> SLLISYESDFKTTLEQAKASLAEAPSQPLSQRNTTLKHVEQQQDELFD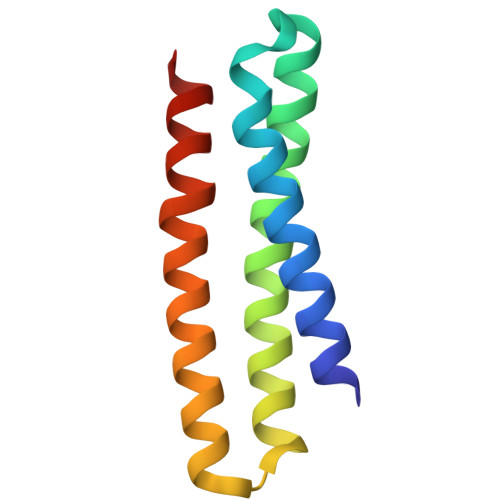LLDQMDVEVNNSIGDASERATYKAKLREWKKTIQSDIKRPLQSLVDSGD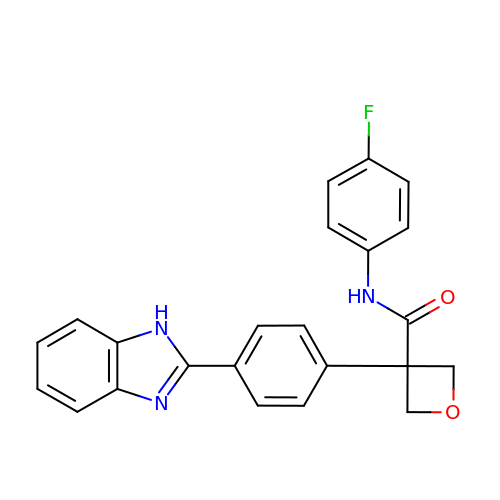3-[4-(1H-benzimidazol-2-yl)phenyl]-N-(4-fluorophenyl)oxetane-3-carboxamide | C23 H18 F N3 O2 | OLDGOAIEJVEZFL-UHFFFAOYSA-N> GSHMSGIALSRLAQERKAWRKDHPFGFVAVPTKNPDGTMNLMNWECAIPGKKGTPWEGGLFKLRMLFKDDYPSSPPKCKFEPPLFHPNVYPSGTVCLSILEEDKDWRPAITIKQILLGIQE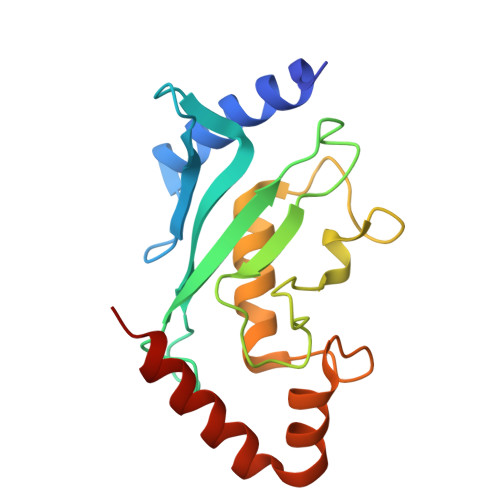LLNEPNIQSPAQAEAYTIYCQNRVEYEKRVRAQAKKFAPS> MSSSENTLLDGKSENTIRFLTFNVNGIRTFFHYQPFSQMNQSLRSVFDFFRADIITFQELKTEKLSISKWGRVDGFYSF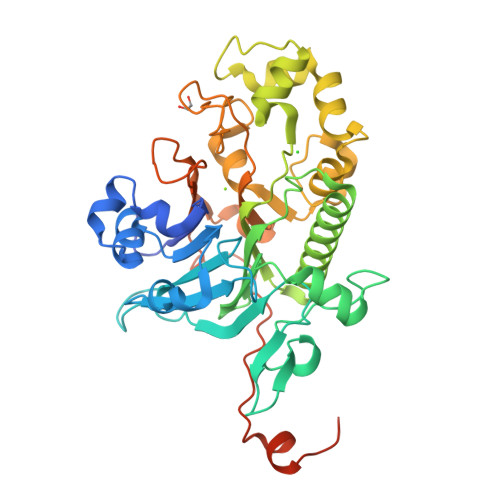ISIPQTRKGYSGVGCWIRIPEKNHPLYHALQVVKAEEGITGYLTIKNGKHSAISYRNDVNQGIGGYDSLDPDLDEKSALELDSEGRCVMVELACGIVIISVYCPANSNSSEEGEMFRLRFLKVLLRRVRNLDKIGKKIVLMGDVNVCRDLIDSADTLEQFSIPITDPMGGTKLEAQYRDKAIQFIINPDTPHRRIFNQILADSLLPDASKRGILIDTTRLIQTRNRLKMYTVWNMLKNLRPSNYGSRIDFILVSLKLERCIKAADILPDILGSDHCPVYSDLDILDDRIEPGTTQVPIPKFEARYKYNLRNHNVLEMFAKKDTNKESNENLYFQ The physiological role of the E. coli ChrR is quinone reductase, and this is likely to be the case for enzymes of this class also in other bacteria. Reductions mediated by ChrR involve electron transfer from NADH to the various substrates via ping-pong bi-bi (double displacement) reaction resulting in the transfer of electrons from NADH to the enzyme bound flavin co-factor, which subsequently passes them on to the enzyme substrate. We discovered the soluble ChrR class of enzymes in search for such a mechanism. This class of enzymes is widely distributed in bacteria, and can greatly mitigate redox cycling not only by a one-step reduction of chromate to Cr(III) but also by preempting its reduction by cellular one-electron reducers. Structurally, ChrR belongs to the FMN reductase family of flavodoxin superfamily.

In order to gain mechanistic insights into this important enzyme, which could afford rational means for its improvement, we report here the crystal structure of the E. coli ChrR enzyme at 2.2 Å resolution. FMN, representing the enzyme active site, is located in a shallow cavity surrounded by loops 1, 3 and 4 at the C-terminus of the β-sheet. FMN is anchored by several hydrogen bonds to a typical strand-loop-helix nucleotide-binding motif GSLRKGSFN (residues 12 to 20) located on loop 1 of the protein. The asymmetric unit is composed of two molecules forming a homo-dimer with a buried surface of 4670 Å2 (about 32%) for a total surface area of 14630 Å2. In the dimer, the two FMN prosthetic groups locate at opposite sides of the interface with loop 2 from one monomer covering the prosthetic group of the other monomer. A potential metal binding site is observed in the dimer interface, involving residues Asn50 and Asp52 (loop 2) from one monomer and the carbonyl oxygen of Leu14 (loop 3) of the other. A calcium ion has been modeled at this site because the crystallization buffer contains calcium. However, size-exclusion chromatography at various protein concentrations, including those used for measuring the enzyme activity, showed that the active enzyme is indeed a tetramer. Within the tetramer, the dimers interact by a pair of two hydrogen bond networks, each involving Tyr128 and Glu146 of one dimer and Arg125 and Tyr85 of the other with the latter extending to one of the redox FMN cofactors, as shown in Fig. 3. We also show that a hydrogen bond network involving four amino acids at the dimer-dimer interface and reaching towards the flavin mononucleotide (FMN) cofactor plays a central role in chromate reductase activity of ChrR.

>[2x]MAEKLQVVTLLGSLRKGSFNGMVARTLPKIAPASMEVNALPSIADIPLYDADVQQEEGFPATVEALAEQIRQADGVVIVTPEYNYSVPGGLKNAIDWLSRLPDQPLAGKPVLIQTSSMGVIGGARCQYHLRQILVFLDAMVMNKPEFMGGVIQNKVDPQTGEVIDQGTLDHLTGQLTAFGEFIQRVKILEGSS>MIKLKNVTKTYKMGEEIIYALKNVNLNIKEGEFVSIMGPSGSGKSTMLNIIGCLDKPTEGEVYIDNIKTNDLDDDELTKIRRDKIGFVFQQFNLIPLLTALENVELPLIFKYRGAMSGEERRKRALECLKMAELEERFANHKPNQLSGGQQQRVAIARALANNPPIILADQPTGALDSKTGEKIMQ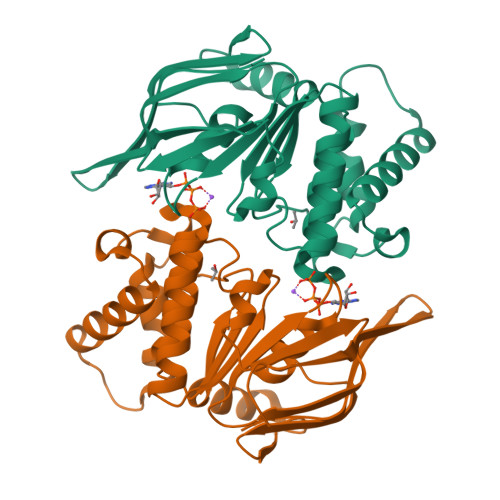LLKKLNEEDGKTVVVVTHDINVARFGERIIYLKDGEVEREEKLRGFDDR[2x]> MGGSHHHHHHLESTSLYKKSSSTPPRGVTVVNNFDAKRYLGTWYEIARFD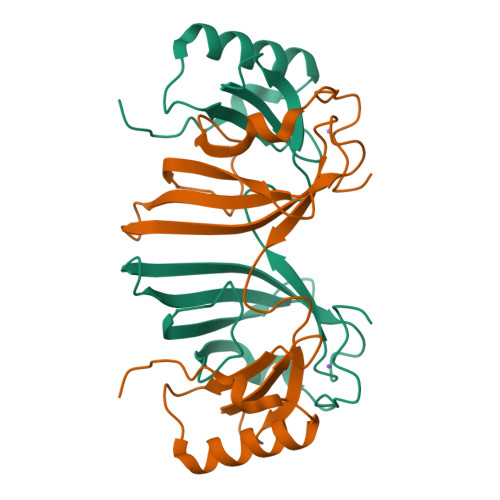HRFERGLEKVTATYSLRDDGGLNFINKGYNPDRGMWQQSEGKAYFTGAPTRAALKVSFFGPFYGGYNVIALDREYRHALVCGPDRDYLWIQSRTPTISDEVKQEMLAVATREGFDVSKFIWVQQPGS>[2x]MKTIIINGVQFNTDEDTTILKFARDNNIDISALCFLNNCNNDINKCEICTVEVEGTGLVTACDTLIEDGMIINTNSDAVNEKIKSRISQLLDIHEFKCGPCNRRENCEFLKLVIKYKARASKPFLPKDKTEYVDERSKSLTVDRTKCLLCGRCVNACGKNTETYAMKFLNKNGKTIIGAEDEKCFDDTNCLLCGQCIIACPVAALSEKSHMDRVKNALNAPEKHVIVAMAPSVRASIGELFNMGFGVDVTGKIYTALRQLGFDKIFDINFGADMTIMEEATALVQRIENNGPFPMFTSCCPGWVRQAENYYPELLNNLSSAKSPQQIFGTASKTYYPSISGLDPKNVFTVTVMPCTSKKFEADRPQMEKDGLRDIDAVITTRELAKMIKDAKIPFAKLEDSEADPAMGEYSGAGAIFGATGGVMEAALRSAKDFAENAELEDIEYKQVRGLNGIKEAEVEINNNKYNVAVINGASNLFKFMKSGMINEKQYHFIEVMACHGGCVNGGGQPHVNPKDLEKVDIKKVRASVLYNQDEHLSKRKSHENTALVKMYQNYFGKPGEGRAHEILHFKYKKSAWSHPQFEK

[FeFe]-hydrogenases represent one of natures’ most effective classes of redox enzymes catalyzing the reversible reduction of protons to dihydrogen (H2) at turnover frequencies of up to 9000 s-11–3. With their low catalytic over-potential, [FeFe]-hydrogenases represent excellent models for a regenerative and likewise economically feasible H2 production. Their active center (“H-cluster”) can be structured into a standard [4Fe-4S]-cluster ([4Fe]H) and a diiron site ([2Fe]H). Theoretical studies suggest that the most probable PT pathway comprises of strictly conserved residues E282, S319, E279, and C299 (from surface to H-cluster, numbering corresponds to CpI), including two protein-bound water molecules (Wat826, Wat1120 4XDC19, chain B) located between E279 and C29915,16,20. In this study, site-directed mutagenesis (SDM) is used to investigate the PT pathway of two [FeFe]-hydrogenases, namely CpI and HydA1, which represent the largest (M3) and smallest (M1) type of monomeric [FeFe]-hydrogenases, respectively.

Corresponding to earlier crystal structure data, for all CpI variants a space group of P1 21 1 was observed with two copies in the asymmetric unit cell (chain A and B). For the same PT pathway position, different substitutions can have a dramatically different impact as exemplified by position E144HydA1/E282CpI. Here the exchange to glutamine diminished enzyme activity to only 0.4–8%, while the non-conservative exchange to alanine and the conservative exchange to aspartic acid retained between 46 and 81% activity. In E282A, two water molecules occupy the space of the missing carboxylic acid group (chain B, Wat717 and Wat974). The distances between these water molecules and the hydroxyl group of S319 are 2.5 and 3.1 Å, respectively. They are close enough to rescue the PT activity between surface water and S319CpI further downstream the PT pathway. As a consequence, Hhyd with its deprotonated adt-NH ligand would be stabilized in presence of H2 (E279A). In case of the corresponding exchange at the surface-exposed glutamate in E282ACpI, two H2O molecules (chain B: Wat717 and Wat974) invading from the solvent are able to bridge the gap of the missing carboxyl group (E282A and Supplementary Fig. 13a) thereby rescuing a large fraction of H2-release activity (~50%). The fact that E282ACpI is rescued by an H2O moiety while in E279ACpI and C299ACpI the gap in the catalytic PT pathway cannot be closed, is probably connected to the superior accessibility at the protein surface and the specific functional requirements (such as e.g. pKa) of the position to be rescued within the PT pathway chain. In case of E282CpI, a substitution for aspartic acid shifted the optimum only slightly to pH 7.5 while an exchange to alanine or glutamine rendered the enzyme most active at pH 7 and 6, respectively.>GLPRVAVDLVAPPLVHPHSQVAAGAPKVVQFRMSIEEKKMVADDDGTTAQAMTFNGSVPGPTLVVHEGDYIELTLVNPATNSMPHNVDFHAATGALGGAGLTQVVPGQEAVLRFKADRSGTFVYHCAPAGMVPWHVVSGMNGALMVLPRDGLRDAAGAALAYDRVYTIGESDLYVPKAADGNYSDYPALASAYADTVAVMRTLTPSHAVFNGAVGALTGANALTAAVGESVLIIHSQANRDSRPHLIGGHGDWVWTTGKFANPPQLNMETWFIPGGSAAAALYTFKQPGTYAYLSHNLIEAMELGAAAQASVEGQWDDDLMTSVAAPGP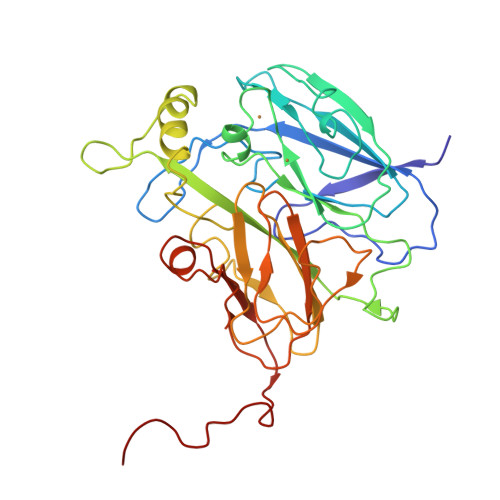A[3x]>[24x]MSNENPIIAINMAKIANKPDSYETMMKVGPKVC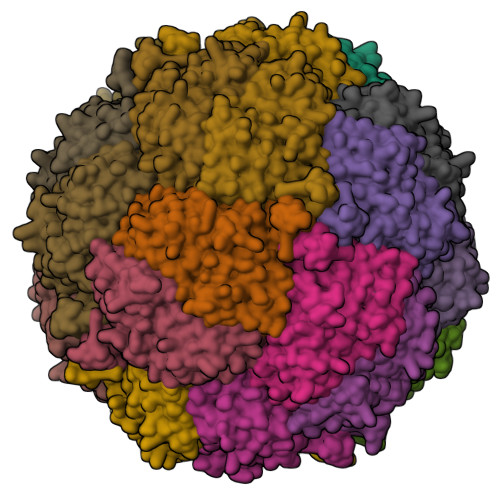ITTASHPGFLGFEQLLQTGIHPMAGRYGGGAVDMRETLNPMGMFQYTVWKDVHSHEEMHHDNFKEIFELCSGCLGMVIEGPWEPYFEVVKSDLPQIMSMTDVPQVLGDSFAKQERVPKVALSSQRTVVIGDHWVMDGHEKAFEQGATETLEWMKANVPGMVGWMIMKQFGVSAIGSFQLDPEGAMKAVSTLGANPPEYNTNYGNKVHDKPPIPGQTPTQYLVHIEWESPEHAHQGLGHVMVDYELRQIHNNGVLAHLDKGPYYMFFSPMMEQGLWRKHLKQ> QQ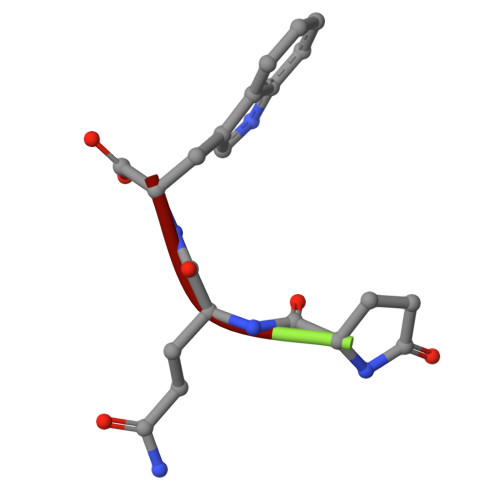W>KDMFNT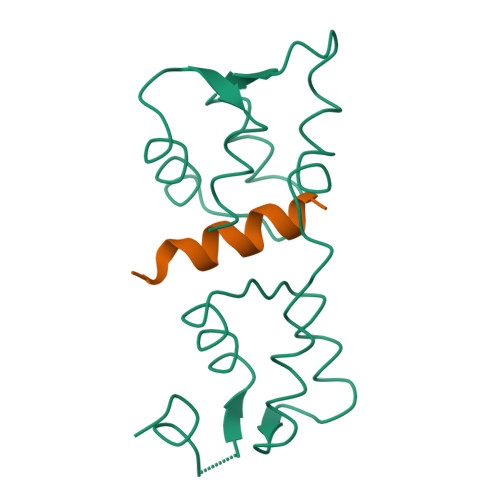KSSNGKLRIEDASHNARKLGLAPSSTDEKKIRDLYGDSLTYEQYLEYLTMCVHDRDNMEELIKMFSHFDNNSSGFLTKNQMKNILTTWGDALTEQEANDALNAFSSEDRINYKLFCEDILS[3x];>[3x]SLMRVQAHIRKRMVA> EQSSSEIKIVRDEYGMPHIYANDTWHLFYGYGYVVAQDRLFQMEMARRSTQGTVAEVL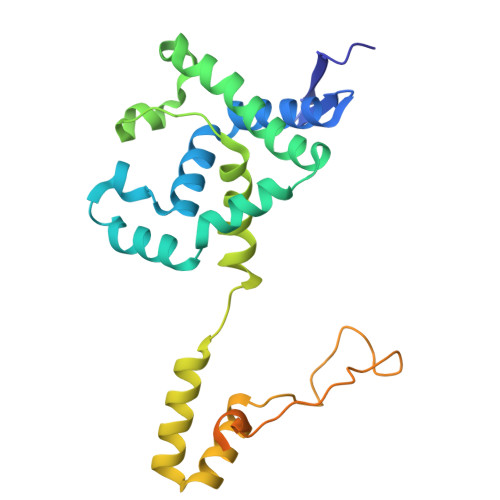GKDFVKFDKDIRRNYWPDAIRAQIAALSPEDMSILQGYADGMNAWIDKVNTNPETLLPKQFNTFGFTPKRWEPFDVAMIFVGTMANRFSDSTSEIDNLALLTALKDKYGVSQGMAVFNQLKWLVNPSAPTTIAVQESNYPLKFNQQNSQTAALLPRYDLPAPMLDRPAKGADGALLALAAGKNRETIAAQFAQGGANGLAGY>GPGSMKLCDFEVGLDQPFFLIAGTCVVESEQMTIDTAGRLKEICEKLNVPFIYKSSYDKANRSSGKSFRGLGMDEGLRILSEVKRQLGLPVLTDVHSIDEIEQVASVVDVLQTPAFLCRQTDFIHACARSGKPVNIKKGQFLAPHDMKNVIDKARDAAREAGLSEDRFMACERGVSFGYNNLVSDMRSLAIMRETNAPVVFDATHSVQLPGGQGTSSGGQREFVPVLARAAVATGVAGLFMETHPNPAEAKSDGPNAVPLNRMGALLETLVTLDQAVKRNPFLENDFN[4x]

Here we report a functional and structural genomics effort that applied saturation-level transposon mutagenesis and next generation sequencing (Tn-seq) to identify essential genes in B. thailandensis, followed by high-throughput structure determination. We used an “ortholog rescue” approach to maximize structural coverage of these gene families, which are likely to be essential not only in B. thailandensis, but also in related, but more virulent, Burkholderia species, such as B. pseudomallei. Using only seven Burkholderia species to select orthologs of essential genes, we solved structures for 49/406 essential gene families, and for 56 total Burkholderia protein targets (including seven ortholog replicates). Of these 56 targets, 25 satisfied criteria for being a potential antimicrobial drug target.

By using an ortholog rescue strategy for insoluble or difficult to crystallize targets, we increased our structural coverage of B. thailandensis essential genes from 31/406 (7.6%) to 49/406 (12.1%). For the seven pairs of ortholog structures (with no bound ligand) solved in this study, the average overall Cα RMSD was 1.5±0.5 Å, indicating a high degree of structural similarity. This structural similarity suggests that the ortholog approach is an efficient method to obtain useable structures from otherwise intractable targets, thereby lowering the barrier to structure-based drug design targeting infectious organisms.> MRGSHHHHHHGSLMPGGKEFYNFYPEYVVGLQWMGDNYVFIEGDDLVFNKANGKSAQTTRFSAADLNALMPEGCKFQTTDAFPSFRTLDAGRGLVVLFTQGGLVGFDMLARKVTYLFDTNEETASLDFSPVGDRVAYVRNHNLYIARGGKLGEGMSRAIAVTIDGTETLVYGQAVHQREFGIEKGTFWSPKGSCLAFYRMDQSMVKPTPIVDYHPLEAESKPLYYPMAGTPSHHVTVGIYHLATGKTVYLQTGEPKEKFLTNLSWSPDENILYVAEVNRAQNECKVNAYDAETGRFVRTLFVETDKHYVEPLHPLTFLPGSNNQFIWQSRRDGWNHLYLYDTTGRLIR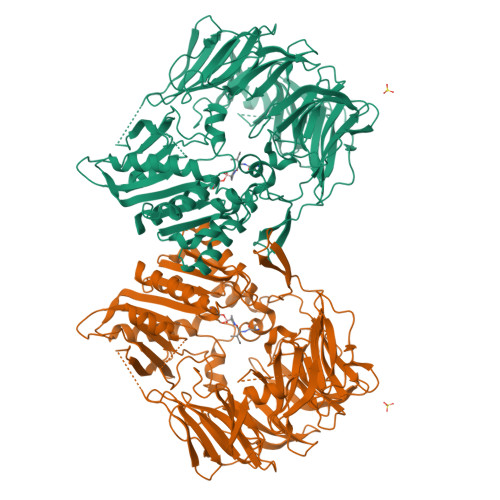QVTKGEWEVTNFAGFDPKGTRLYFESTEASPLERHFYCIDIKGGKTKDLTPESGMHRTQLSPDGSAIIDIFQSPTVPRKVTVTNIGKGSHTLLEAKNPDTGYAMPEIRTGTIMAADGQTPLYYKLTMPLHFDPAKKYPVIVYVYGGPHAQLVTKTWRSSVGGWDIYMAQKGYAVFTVDSRGSANRGAAFEQVIHRRLGQTEMADQMCGVDFLKSQSWVDADRIGVHGWSYGGFMTTNLMLTHGDVFKVGVAGGPVIDWNRYEIMYGERYFDAPQENPEGYDAANLLKRAGDLKGRLMLIHGAIDPVVVWQHSLLFLDACVKARTYPDYYVYPSHEHNVMGPDRVHLYETITRYFTDHL Spiroviolene synthase (SvS) from Streptomyces violens was first described by Rabe et al. and represents a bacterial class I diterpene cyclase that we were not able to produce in sufficient quantities for crystallization due to protein instability. Terpene cyclases such as SvS form a variety of complex multicyclic compounds with potent biological activities via carbocationic, electrophilic cyclization cascades of relatively simple substrates, either by metal-ion assisted release of an allylic pyrophosphate (class I mechanism) or by protonation of an oxirane/ene-functionality (class II mechanism). We previously reported a hypothetical ancestor of SvS—SvS-A2 26—which shares 77% sequence identity with the extant enzyme.

In particular, we noticed a surface patch of five consecutive ancestral mutations (205DREMH209) in the turn directly preceding helix H. This patch is located 17.9 Å away from the carbonyl atom of the effector residue (Ala186), so that it unlikely impacts the activity of SvS-A2. Moreover position 89 in the catalytic DDxx(x)D motif occupies a His in SvS-WT, but an Ala on the surface of SvS-A2. Exchanging these six residues on the surface back to the corresponding wild-type residues (205–209:DREMH/AQDLE and Ala89His) resulted in a surface variant of SvS-A2 with similar stability, despite an overall reduced expression yield. Therefore, we anticipated that the surface variant may constitute a more suitable structural template for homology modeling of SvS-WT, especially with respect to adequately capturing substrate binding. Using the surface variant as a template (monomeric with modeled loops, metal cluster and GGPP) resulted in a homology model (SvS-WT-Hom2) with overall higher sequence identity as well as optimal average scores for dihedral angles (Z-score of +0.541). Specifically, the local Z-score slightly improved for the catalytic DDxx(x)D and NSE motifs (arrows), even though the local Z-score for the RY-dimer decreased. Overall, we considered the homology model derived from the SvS-A2 surface variant (SvS-WT-Hom2) more suitable for mechanistic analysis of the extant enzyme. Redesigning the surface of the ancestral enzyme to restore wild-type sequence at selected positions provided a crystal structure representing an optimized template and improved the confidence in the derived homology model of the extant enzyme, in particular for regions involved in substrate and cofactor binding.

>[2x]MAMTVTEVDLPPIYCPLESAIHPRVHEVEKRAVEWIRRSGMCASEEERAWVIATHSADFFARFAPTAADEDRLLATSLWVYWGFAFDDHRCDNGPLSTRPAQFNALAGRVQRALEAPSAEDNGDRFVPALQDIARRFRSFGTPTQVRRFVHAHRAWLSGVAWQIGNQARGHMPGLDDYLAMRLLSAGGEPTFAMLEIATGAEVPAQDLERPAVRALTEMAIMVAALDNDRHSLRKELSRGHTDQNIYSVLMHHRGMSLQEAVEEATKLRDRILLRFLELHDRVRPGAGAELSTYLQGLRHGIRGNAEWGLRVPRYLSLGRVPDPMEDAPLTWAESPSDSSPSPLPGAPSIAWWWDDALLGA>[2x]IETVEFRVTGTTRRSYSDFLQNLRNRLSSGTSVHDIPLLPAQSGSQQDLLFVRLFDWGNRPITLVLNRVNAYVVAYQAQNRFYLLSDTPANPQVYGNNPHRLTFTGSYGALQNVAKSNRENIDLGINPLATAITTLHNW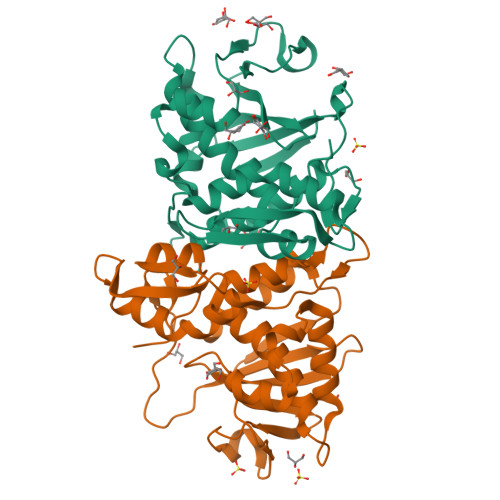SPPTVETSVARSLIVLIQLVSETARFRAIEQRVTNNIIDQVTPIRYDNFRPRVGIIDLQTNWQTLSTEVQRAEGGRFLQPVKLQVSVQQTVVISDVEKARTFCGLALLLRWRPSQASLSSHDFAWRDIRSILDIGA>[4x]MSLIIQVSPAGSMDLLSQLEVERLKKTASSDLYQLYRNCSLAVL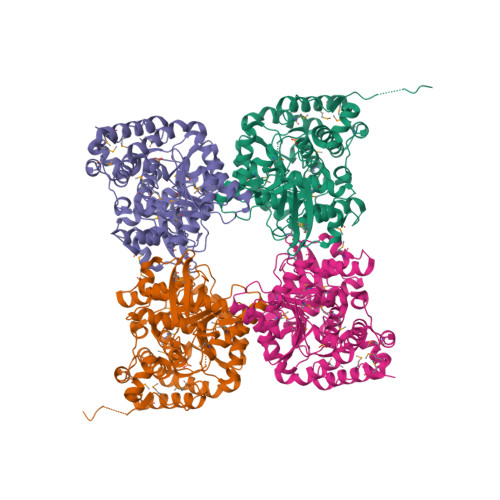NSGSHTDNSKELLDKYKNFDITVMRRERGIKLELANPPEHAFVDGQIIKGIQEHLFSVLRDIVYVNMHLADSQRLNLTNATHITNLVFGILRNAGALIPGATPNLVVCWGGHSINEVEYQYTREVGHELGLRELNICTGCGPGAMEGPMKGAAVGHAKQRYSEYRYLGLTEPSIIAAEPPNPIVNELVIMPDIEKRLEAFVRMAHGIIIFPGGPGTAEELLYILGIMMHPENADQPMPIVLTGPKQSEAYFRSLDKFITDTLGEAARKHYSIAIDNPAEAARIMSNAMPLVRQHRKDKEDAYSFNWSLKIEPEFQLPFEPNHESMANLDLHLNQRPEVLAANLRRAFSGVVAGNVKAEGIREIERHGPFEMHGDPVLMKKMDQLLNDFVAQNRMKLPGGSAYEPCYKIVTEGHHHHHH> GSEANYRKDFIDTMTRELYDAFLHERLYLIYMDSRAELKRNSTLKKKFF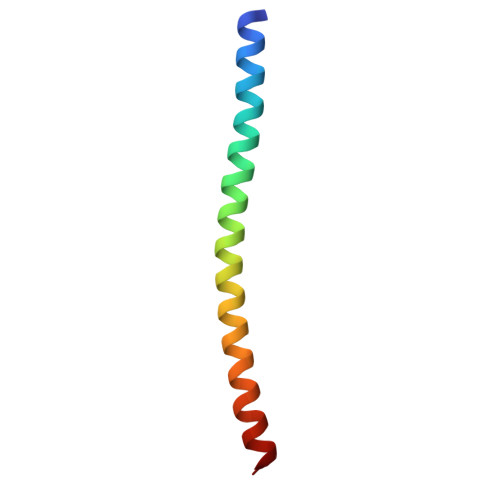EKWQAS>[2x]MRLWKAVVVTLAFVSTDVGVTTAIYAFSHLDRSLLEDIRHFNIFDSVLDLWAACLYRSCLLLGATIGVAKNSALGPRRLRASWLVITLVCLFVGIYAMAKLLLFSEVRRP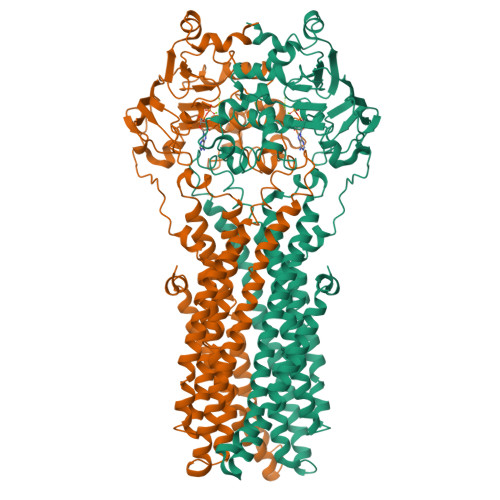IRDPWFWALFVWTYISLAASFLLWGLLATVRPDAEALEPGNEGFHGEGGAPAEQASGATLQKLLSYTKPDVAFLVAASFFLIVAALGETFLPYYTGRAIDSIVIQKSMDQFTTAVVVVCLLAIGSSLAAGIRGGIFTLVFARLNIRLRNCLFRSLVSQETSFFDENRTGDLISRLTSDTTMVSDLVSQNINIFLRNTVKVTGVVVFMFSLSWQLSLVTFMGFPIIMMVSNIYGKYYKRLSKEVQSALARASTTAEETISAMKTVRSFANEEEEAEVFLRKLQQVYKLNRKEAAAYMSYVWGSGLTLLVVQVSILYYGGHLVISGQMSSGNLIAFIIYEFVLGDCMESVGSVYSGLMQGVGAAEKVFEFIDRQPTMVHDGSLAPDHLEGRVDFENVTFTYRTRPHTQVLQNVSFSLSPGKVTALVGPSGSGKSSCVNILENFYPLQGGRVLLDGKPIGAYDHKYLHRVISLVSQEPVLFARSITDNISYGLPTVPFEMVVEAAQKANAHGFIMELQDGYSTETGEKGAQLSGGQKQRVAMARALVRNPPVLILDEATSALDAESEYLIQQAIHGNLQRHTVLIIAHRLSTVERAHLIVVLDKGRVVQQGTHQQLLAQGGLYAKLVQRQMLGLEHPLDYTASHKEPPSNTEHKA>[6x]AAGMYLEHYLDSIENLPFELQRNFQLMRDLDQRTEDLKAEIDKLATEYMSSARSL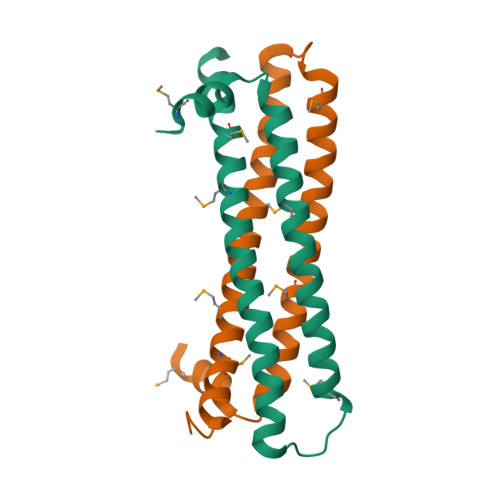SSEEKLALLKQIQEAYGKCKEFGDDKVQLAMQTYEMVDKHIRRLDTDLA> HMRKKIFKPEELRQALMPTLEALYRQDPESLPFRQPVDPQLLGIPDYFDIVKNP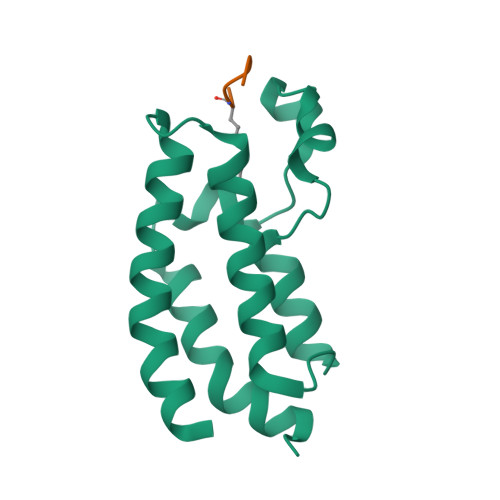MDLSTIKRKLDTGQYQEPWQYVDDVWLMFNNAWLYNRKTSRVYKFCSKLAEVFEQEIDPVMQSL;> GTVALREIRRYQKS>[2x]GAMAQNITARIGEPLVLKCKGAPKKPPQRLEWKLNTGRTEAWKVLSPQGGGPWDSVARVLPNGSLFLPAVGIQDE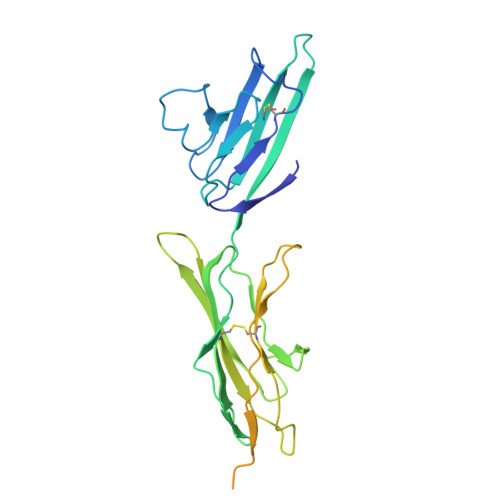GIFRCQAMNRNGKETKSNYRVRVYQIPGKPEIVDSASELTAGVPNKVGTCVSEGSYPAGTLSWHLDGKPLVPNEKGVSVKEQTRRHPETGLFTLQSELMVTPARGGDPRPTFSCSFSPGLPRHRALRTAPIQPRVWEPVPLEEVQLVVEPEGGAVAPGGTVTLTCEVPAQPSPQIHWMKDGVPLPLPPSPVLILPEIGPQDQGTYSCVATHSSHGPQESRAVSISIIEP>[4x]GSSPEKPTPNGGIPHDNLVLIRMKPDENGRFGFNVKGGYDQKMPVIVSRVAPGTPADLCVPRLNEGDQVVLINGRDIAEHTHDQVVLF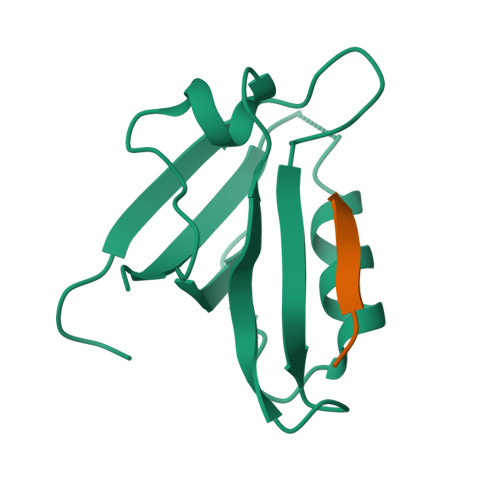IKASCERHSGELMLLVRPN;>[4x]SWARVSKETPL> MQELYLLGVVPSRRFEAVVNSLSKTLDGPKTILEFWVVYRPKDVPPNLPRQPDSWLRLCSNIESHDETDTEWSKNTQWSMYLE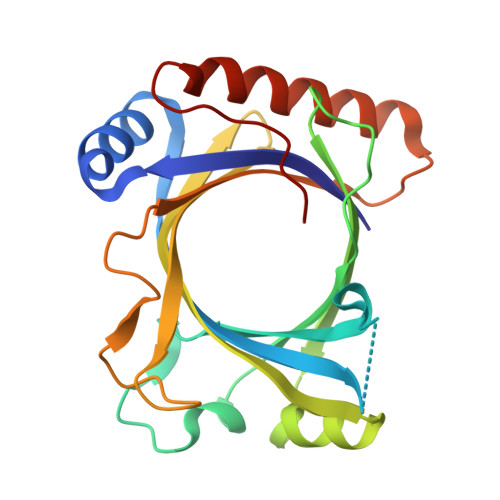GNSEPKREDKCGIRPVNRAKLTNGSVTEFVEKMGYEFSHEYIIQGLEYFFFDTTVRIYQTLIPSQQRSIKPPFHPMNEEQPWILHVYTHVADASNQVAMAKAEANLTKVKTLLSAFCDLKNVRL>[2x]MSTQYETQGYTINNAGRRLVVDPITRIEGHMRCEVNINDQNVITNAVSCGTMFRGLEIILQGRDPRDAWAFVERICGVCTGVHALASVYAIEDAIGIKVPDNANIIRNIMLATLWCHDHLVHFYQLAGMDWIDVLDALKADPRKTSELAQSLSSWPKSSPGYFFDVQNRLKKFVEGGQLGIFRNGYWGHPQYKLPPEANLMGFAHYLEALDFQREIVKIHAVFGGKNPHPNWIVGGMPCAINIDESGAVGAVNMERLNLVQSIITRTADFINNVMIPDALAIGQFNKPWSEIGTGLSDKCVLSYGAFPDIANDFGEKSLLMPGGAVINGDFNNVLPVDLVDPQQVQEFVDHAWYRYPNDQVGRHP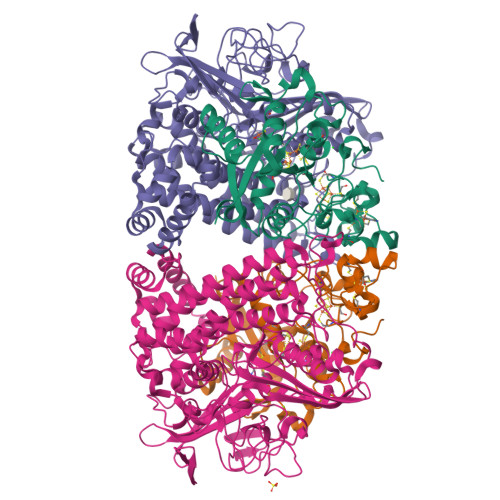FDGITDPWYNPGDVKGSDTNIQQLNEQERYSWIKAPRWRGNAMEVGPLARTLIAYHKGDAATVESVDRMMSALNLPLSGIQSTLGRILCRAHEAQWAAGKLQYFFDKLMTNLKNGNLATASTEKWEPATWPTECRGVGFTEAPRGALGHWAAIRDGKIDLYQCVVPTTWNASPRDPKGQIGAYEAALMNTKMAIPEQPLEILRTLHSFDPCLACSTH;>[2x]KPRIPVVWIHGLECTCCTESFIRSAHPLAKDVILSLISLDYDDTLMAAAGTQAEEVFEDIITQYNGKYILAVEGNPPLGEQGMFCISSGRPFIEKLKRAAAGASAIIAWGTCASWGCVQAARPNPTQATPIDKVITDKPIIKVPGCPPIPDVMSAIITYMVTFDRLPDVDRMGRPLMFYGQRIHDKCYRRAHFDAGEFVQSWDDDAARKGYCLYKMGCKGPCTYNACSSTRWNDGVSFPIQSGHGCLGCAENGFWDRGSFYSRVVDIPQMGTHSTADTVGLTALGVVAAAVGVHAVASAVDQRRRHNQQPTETEHQPGNEDKQA>GSMADLDDIKDGKDFRTDQPQKNIPFTLKGCGALDWGMQSRLSRIFNPKTGKTVMLAFDHGYFQGPTTGLERIDINIAPLFEHADVLMCTRGILRSVVPPATNRPVVLRASGANSILAELSNEAVALSMDDAVR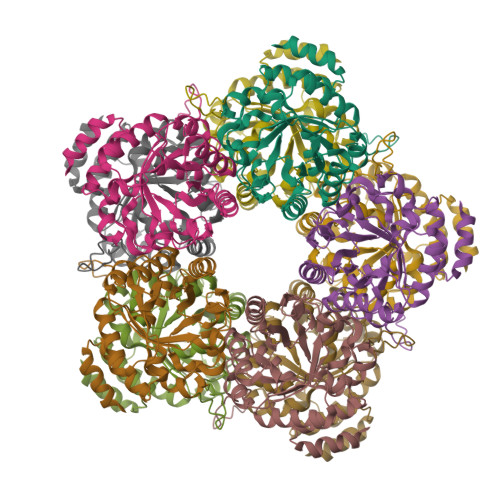LNSCAVAAQVYIGSEYEHQSIKNIIQLVDAGMKVGMPTMAVTGVGKDMVRDQRYFSLATRIAAEMGAQIIKTYYVEKGFERIVAGCPVPIVIAGGKKLPEREALEMCWQAIDQGASGVDMGRNIFQSDHPVAMMKAVQAVVHHNETADRAYELYLSEKQ[20x]>[4x]MPVRRGHVAPQNTFLDTIIRKFEGQSRKFIIANARVENCAVIYCNDGFCELCGYSRAEVMQRPCTCDFLHGPRTQRRAAAQIAQALLGAEERKVEIAFYRKDGSCFLCLVDVVPVKNEDGAVIMFILNFEVVMEKDMVGSSPTSDREIIAPKIKERTHNVTEKVTQVLSLGADVLPEYKLQAPRIHRWTILHYSPFKAVWDWLILLLVIYTAVFTPYSAAFLLKETEEGPPATECGYACQPLAVVDLIVDIMFIVDILINFRTTYVNANEEVVSHPGRIAVHYFKGWFLIDMVAAIPFDLLIFGSGSEELIGLLKTARLLRL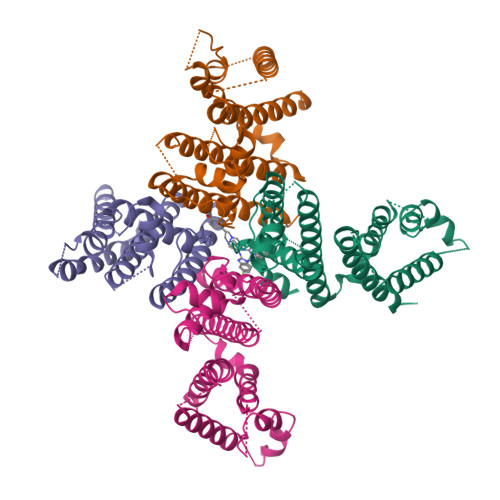VRVARKLDRYSEYGAAVLFLLMCTFALIAHWLACIWYAIGNMEQPHMDSRIGWLHNLGDQIGKPYNSSGLGGPSIKDKYVTALYFTFSSLTSVGFGNVSPNTNSEKIFSICVMLIGSLMYASIFGNVSAIIQRLYSGTARYHTQMLRVREFIRFHQIPNPLRQRLEEYFQHAWSYTNGIDMNAVLKGFPECLQADICLHLNRSLLQHCKPFRGATKGCLRALAMKFKTTHAPPGDTLVHAGDLLTALYFISRGSIEILRGDVVVAILGKNDIFGEPLNLYARPGKSNGDVRALTYCDLHKIHRDDLLEVLDMYPEFSDHFWSSLEITFNLRDTNMIPGGRQYQELPRCPAPTPSLLNIPLSSPGRRPRGDVESRLDALQRQLNRLETRLSADMATVLQLLQRQMTLVPPAYSAVTTPGPGPTSTSPLLPVSPLPTLTLDSLSQVSQFMACEELPPGAPELPQEGPTRRLSLPGQLGALTSQPLHRHGSDPGSLEVLFQ>[2x]SNAMKQTELLKGILEGL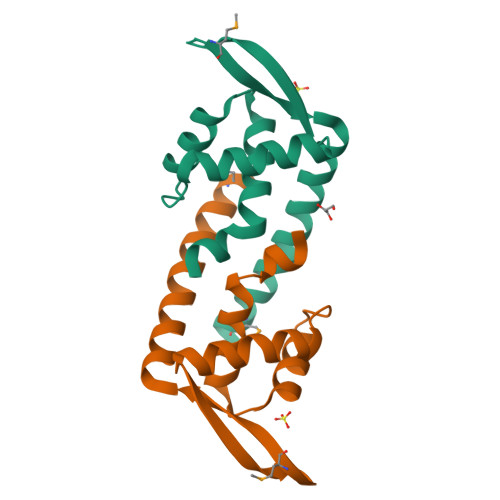VLAIIQRKETYGYEITKILNDQGFTEIVEGTVYTILLRLEKNQWVIAEKKPSEKGPMRKFYRLTSSGEAELADFWQRWTLLSKQVNKMKKNGGIEHVKF>MKIIILGAGQVGGTLAENLVGENNDITIVDNNADRLRELQDKYDLRVVNGHASHPDVLHEAGAQDADMLVAVTNTDETNMAACQVAFTLFNTPNRVARIRSPEYLAEKEALFKSGAIPVDHLIAPEELVTSYIERLIQYPGALQVVSFAEQKVSLVAVKAYYGGPLVGNALSALREHMPHIDTRVAAIFRQGRP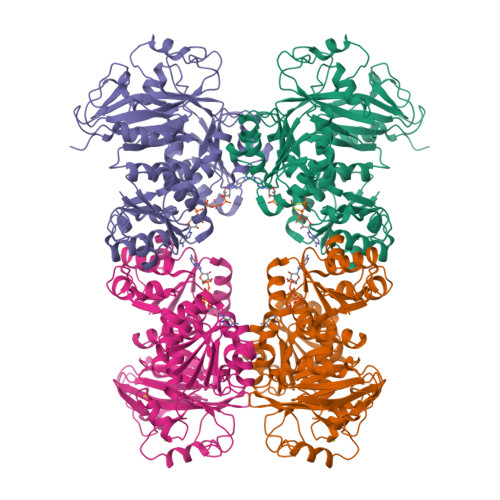IRPQGTTIIEADDEVFFVAASNHIRSVMSELQRLEKPYRRIMIVGGGNIGASLAKRLEQTYSVKLIERDYQRAEKLSEQLENTIVFCGDAADQELLTEENIDQVDVFIALTNEDETNIMSAMLAKRMGAKKVMVLIQRGAYVDLVQGGVIDVAISPQQATISALLTHVRRADIVNVSSLRRGAAEAIEAVAHGDETTSKVVGRAIGDIKLPPGTTIGAVVRGEEVLIAHDRTVIEQDDHVVMFLVDKKYVPDVEALFQPSPFFL[2x]> APQQGTNVNDKVHFSNIDIAIDKGHVNQTTGKTEFWATSSDVLKLKANYTIDDSVKEGDTFTFKYGQYFRPGSVRLPSQTQNLYNAQGNIIAKGIYDSTTNTTTYTFTNYVDQYTNVRGSFEQVAFAKRKNATTDKTAYKMEVTLGNDTYSEEIIVDYGNKKAQPLISSTNYINNEDLSRNMTAYVNQPKNTYTKQTFVTNLTGYKFNPNAKNFKIYEVTDQNQFVDSFTPDTSKLKDVTDQFDVIYSNDNKTATVDLMKGQTSSN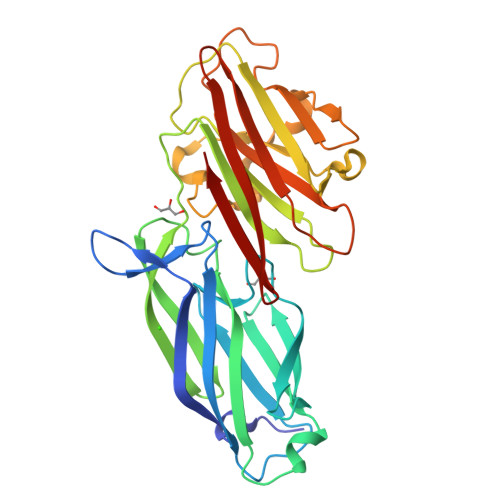KQYIIQQVAYPDNSSTDNGKIDYTLDTDKTKYSWSNSYSNVNGSSTANGDQKK> MGSSHHHHHHSSGRENLYFQGMKSITFEEHYVIEDIQKETMNAISADPKGVPMKVMLEGLEKKTGFTNADELSHHDERIQFMNNQDVQIQVLSYGNGSPSNLVGQKAIELCQKANDQLANYIAQYPNRFVGFATLPINEPEAAAREFERCINDLGFKGALIMGRAQDGFLDQDKYDIIFKTAENLDVPIYLHPAPVNSDIYQSYYKGNYPEVTAATFACFGYGWHIDVGIHAIHLVLSGIFDRYPKLNMIIGHWGEFIPFFLERMDEALFAEHLNHSVSYYFKNSFYITPSGMLTKPQ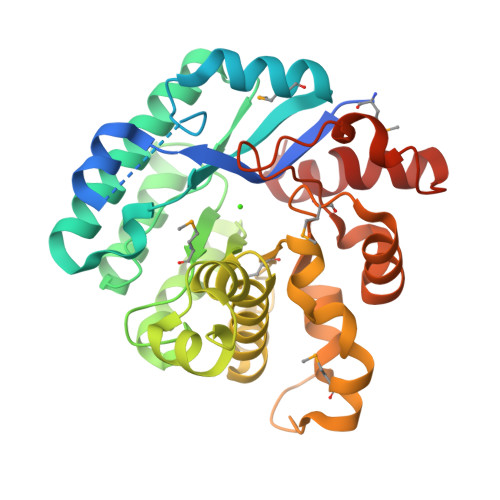FDLVKKEVGIDRILYAADYPYIEPEKLGVFLDELGLTDEEKEKISYTNGAKLLGLSSNN> GMLTYQVKQGDT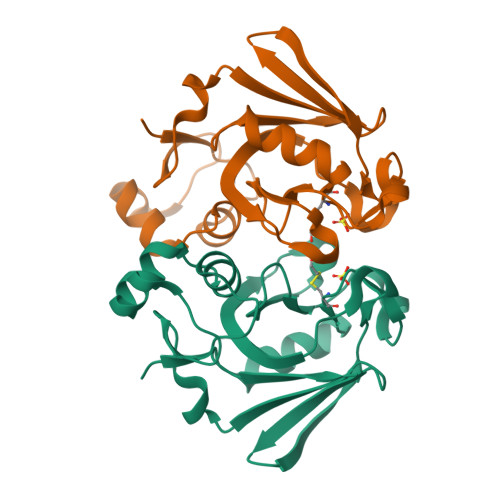LNSIAADFRISTAALLQANPSLQAGLTAGQSIVIPGLPDPYTIPYHIAVSIGAKTLTLSLNNRVMKTYPIAVGKILTQTPTGEFYIINRQRNPGGPFGAYWLSLSAAHYGIHGTNNPASIGKAVSKGCIRMHNKDVIELASIVPNGTRVTINR>[2x]GSFTMNLNFSLLDEPIPLRGGTILVLEDVCVFSKIVQYCYQYEEDSELKFFDHKMKTIKESEIMLVTDILGFDVNSSTILKLIHADLES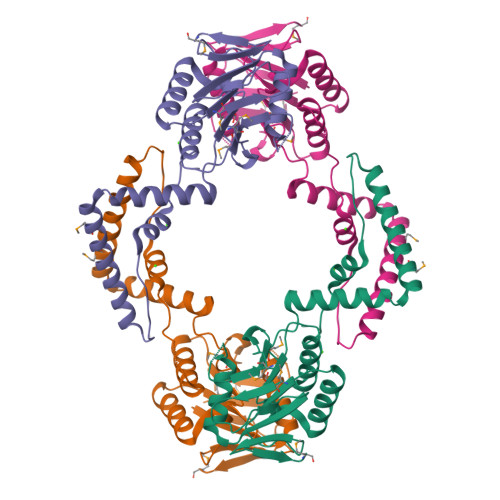QFNEKPEVKSMIDKLVATITELIVFECLENELDLEYDEITILELIKSLGVKVETQSDTIFEKCLEILQIFKYLTKKKLLIFVNSGAFLTKDEVASLQEYISLTNLTVLFLEPRELYDFPQYILDEDYFLITKNMV>[2x]LTEIEHLVQSVCKSYRETCQLRLEDLLRQRSNIFSREEVTGYQRKSMWEMWERCAHHLTEAIQYVVEF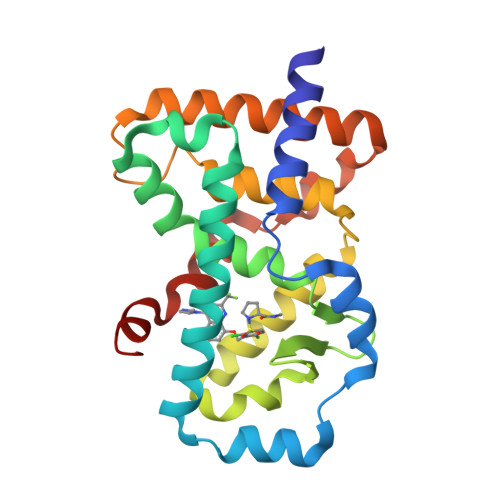AKRLSGFMELCQNDQIVLLKAGAMEVVLVRMCRAYNADNRTVFFEGKYGGMELFRALGCSELISSIFDFSHSLSALHFSEDEIALYTALVLINAHRPGLQEKRKVEQLQYNLELAFHHHLCKTHRQSILAKLPPKGKLRSLCSQHVERLQIFQ> ELNXLLGR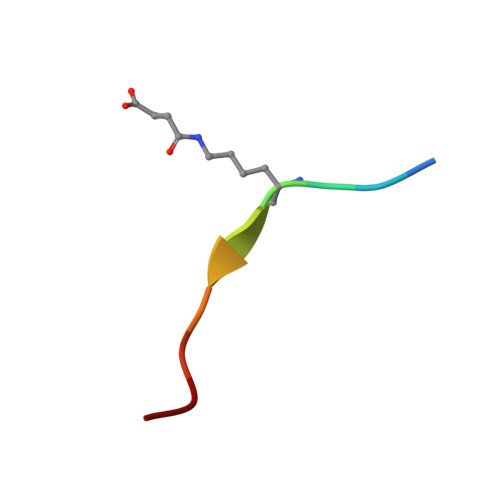VT> MIIDLSQLPEPEVIENLDFETIYQELLGDFREAMAGEWTAEVESDPVLKLLQLAAYRELLLRARINDAARAVMLAYASGADLDQIGAGFNVQRLLIRPAQPEAVPPVEAQ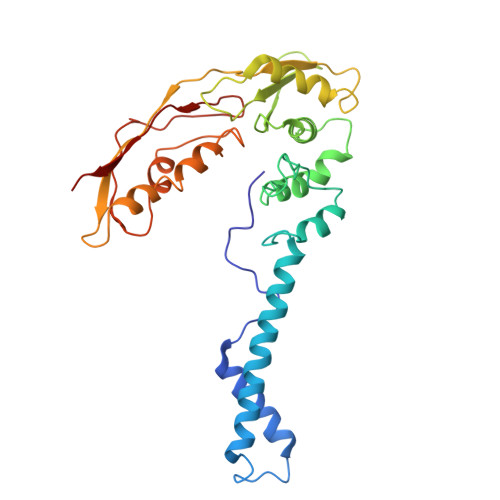YESDKSLRNRIQLAFEQLSVAGPRNAYIAHALGADGRVADASATSPAPCEVLISVLGVEGNGQAPEAVLQAVRLALNAEDVRPVADRVTVRSAGIVPYQVKAQLYLFPGPEAELIRAAAEASLRDYISAQRRLGRDIRRSALFATLHVEGVQRVELQEPAADVVLDETQAAYCTGYAITLGGVDE> HIEGYECQPIFLNVLEAIEPGVVCAGHDNNQPDSFAALLSSLNELGERQLVHVVKWAKALPGFRNLHVDDQMAVIQYSWMGLMVFAMGWRSFTNVNSRMLYFAPDLVFNEYRMHKSRMYSQCVRMRHLSQEFGWLQITPQEFLCMKALL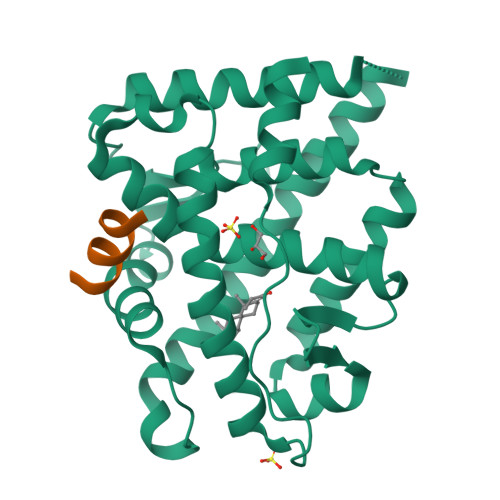LFSIIPVDGLKNQKFFDELRMNYIKELDRIIACKRKNPTSCSRRFYQLTKLLDSVQPIARELYQFTFDLLIKSHMVSVDFPEMMAEIISVQVPKILSGKVKPIYFHTQ;> RGAFQNLFQSV>GSTESFTRRERLRLRRDFLLIFKEGKSLQNEYFVVLFRKNGLDYSRLGIVVKRKFGKATRRNKLKRWVREIFRRNKGVIPKGFDIVVIPRKKLSE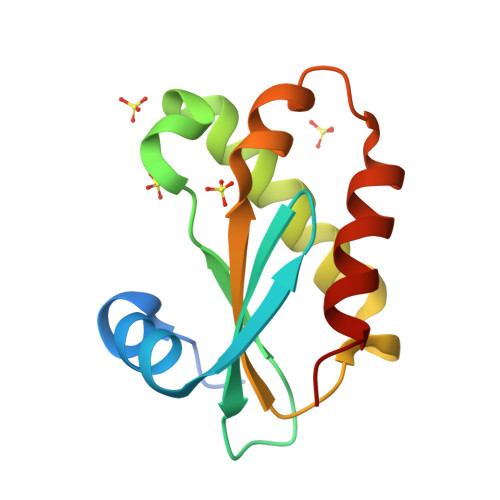EFERVDFWTVREKLLNLLKRIEG[4x]Here, we generated a novel vaccine platform, CTB-V2c, by scaffolding a mucosal-targeting, pentameric particle approaching the size of a typical virus-like particle (VLP) from cholera toxin B (CTB) onto the SIV V2c B-cell epitope, favoring an α-helical conformation of V2. An additional study in macaques demonstrated that V1-deleted (ΔV1) SIV envelope immunogens expose the spike-apical V2 region in an α-helical conformation (designated V2c) and elicit anti-V2c Abs mediating potent ADCC and correlating with decreased risk of SIVmac251 acquisition. Significantly, V2c includes peptide positions 164 to 181 (based on HXBC2 strain numbering), which were targeted for immune selection in the human vaccinees of RV144 (25). We hypothesized that V2c, in isolation from the rest of the HIV/SIV envelope, could elicit functional, non-neutralizing Abs that contribute to vaccine efficacy.

Accordingly, we designed a V2c SIVsmE543-based peptide with the sequence DKKIEYNETWYSRD and scaffolded it on cholera toxin subunit B (CTB-V2c). V2c structural analysis predicted the peptide would take an α-helical conformation and suggested its potential to be stable in vivo. We expressed CTB-V2c in E. coli and purified it by galactose affinity chromatography to select for stable CTB pentamers, as these are the only CTB forms that bind to galactose and mucosal GM1 gangliosides. Moreover, purification of the immunogen also removed endotoxins, which do not bind galactose resin. Gel filtration revealed a pure pentameric fraction of this CTB-V2c chimeric vaccine immunogen. Liquid chromatography-mass spectrometry (LC-MS) confirmed the composition of the molecule, and crystallographic resolution of the structure confirmed a pure, stable pentamer with a dynamic C-terminal peptide insert, consistent with a flexible α-helix DKKIEYNETWYSRD peaked six weeks following the first immunization. Taken together, these data suggested that our CTB-V2c vaccine was successfully immunogenic. Point mutations in the V2c peptide probe revealed that the reactivity of polyclonal sera was dependent on amino acid Y177 within the V2 loop (HXBC2 numbering), which is an amino acid conserved between HIV and SIV viruses and is indispensable for CH58 binding to its B-cell epitope. Indeed, the polyclonal serum Abs elicited by our V2c design were dependent on the V2 loop amino acid Y177, which suggests a focused elicitation in vivo of CH58/CAP228-like, non-neutralizing antibodies in isolation from any other distracting, anti-HIV/SIV Abs. The 5xCTB-V2c/alum group showed no neutralizing antibody responses, suggesting, as suspected, that V2c is not a neutralization epitope.

>[10x]TPQNITDLCAEYHNTQIHTLNDKIFSYTESLAGKREMAIITFKNGATFQVEVPGSQHIDSQKKAIERMKDTLRIAYLTEAKVEKLCVWNNKTPHAIAAISMANDKKIEYNETWYSRD> MSQLQTSLTVIGAGL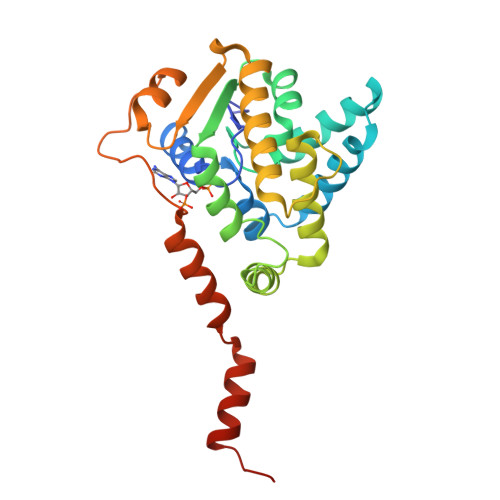PRTGTLSMKKALETIYCQPCYHMYEIILNKQYDISKWQTLLDIKQSKTTSNEILIIQNSLKEILNGYIAVTDLPACGFYRELMTMYPNAKVILTIRDRNDWLTSFRKVVLPRTNDTYKEEVDKVNRILGLNTEFDKMNIDSLKFTFQNNQIDFDDDNNLLECYDEYNKTVQEIVPSERLLVHKLGDGWEPLCQFLNVNIPIGITYPHVNALKEVTELTELLIKYQSLDVIKTKLSEVFGSHHHHHHHH>[2x]MAAQLALNSEASLWGPYREIWQTVLSALIKRQPEAVHSLDIVLKKYKPDFISLFKNPPKSAQQHERVQKASTEGIPIKGTQRTRILEEQLIKEAFILSDLYNIGEIAAVELLLIGEQQQPTFHGLTRGLVAILLYWDGKSCMAESLLHLIQARKGKTFTLDHSPEVVSMVTRFTDDLMEQGLTNKILTLISQIDVNNEFDKLKKERGLGNKKHRKEVSDLIKECQQSLAHSLYSWSCQTPLNREDTLLLIGYLEKVTVEGDGSLDKVNLTLLMSLLYCLDVGFLEQGTDDREELMKQASMFMDRQYIAAIHNRLQNTQPWKSPGMQATVRLAWALALRGISQFSEVLEFSEADEPMAEIAIGGNVFLFLTEAVVGSESFCTDEFFIRRIHKLVTDFPTLMPMKVKQLRNRAEEDARLIQMSMQMGNEPPASLRRDLEHLLLLIGELYRKDPFHLELALEYWCPTEPLQSTSLMGSFLGVAHQRPPQRQVLLSKFVRQMSDLLPATLYLPYLKMLRGLASGPQCAHYCFSLLKANGGSSAENLQAAGGSPVSWDHFFHSLMLYHEHLRRDLPNTDNIHQRHPPLRGITQRELDGLIACLQLTCTIIDWSESARLALCEHAQWMPVVVILGLLQCSIPPLLKAELLKTLAAFGKSPEIAASLWQSLEYTQILQTVRATGLRQGVGIEVELNEIESRCEEYPLTRAFCQLISTLVESSFPTNLGAGLRAPGFEPYLQFLRDTVFLRYRTRAYRRAAEKWEVAEAVLDVFYKLLKDYEPQPEDFVDQYVELQGEERVAFKPPGFSLMHHLLNESPMLELCLSLMEEGVTQLDTYAPFPGKKHLEKAVAYCFMLLNLTLQKENRFMDLLRESHLSMIVTPLEQLLQGINPRSKKADNVVNIARYLCHGNSNAELAFESAKILCSISCNSKIQEKIVGDFTQDQNVSQKLMVGFVSCLDSEEAEELLDSEKEAEDQVKQTNIRYMTKIHILNLLITSLEMKAPNLAMFLLGYELKKPVSTTNLQDSGVLGCPRTCLHSILDILRKGTDVRAGPVAVWDTPHLAELCYQVIYQLCACADTSGPTMRYLRTSQDFLFSQLQHLPFSVEESEISAMNQMSWLMKTATIELRITSLNRQRSHTQRLLHLLLDDMPTRPYSADGEGGMEDESRSLSGFLHFDTTSKVRRKILRILDSIQFSNEIPEPLQLDFFDRSQIEQVIANCEHKNRRGQTVCNVKLLHRVLVAEVNALQGMAAIGQRPLLMEEINTILQYVVERNKLLQCLHAKRHALESWRQLVEIILTACPQDLIPTEHRQLIIRDLLQDLHVKILDDDAAQELMPIVAGAVFTLTAHLSQSVRTELKQPMTASGLGQSQYVQMLDGSFAAPPGTENISAGFASIGDSSLHMILRNLLEFILKTGGGFQRVRAHLYGSLLYYLQIAQRPDEPDTLESAHKSMWERLTAPEDVFSKLQRDNLSIFESYGTALMEVVCRDACDGHDIGRMLALALLDRIVSVDRQQQWLLYLSNSGYLKVLVDSLAEDDVVLRNLLTPQPPLLKALYIYESKMAFLTRVAKSSQGAIELLRSGVIVRLAQCQVYDMRPETDPHGVFGMRETPVFIPAPVERYRQILLPALQICQLILTSSTAQHLQAAGQVLQFLVAHSDTIQAILRSQEGSLGSLQELALLTGIISKAALPGVLNELDIGLNDGSMMELQGHIGRFQRQCLALLNRFGGSDRLRQLSLQDDSSRLDGVSKKDDMELAMQQICSNVMEYCQALMIQNSPSFQQTVCLFTPSLKESASRDGTRQDSQVSILPSWRLPSLGVVIHLLKQSANNFFTYYDIHRQSVGKLQNVEQLPPDEIKELCQSEMPVGADKISTTQKYGLARRRLVKLINSRAKLLSLCSYIIETCLYILWRHLEYYLLHCTTSDSQDPVFSNMTFGNRRFQDTFNTDPNMDPRNLRQNKVSQQDVDTLLREGANSFGESLQKRLLDIESLYCKVRSRHSFIQALVRRIRGLLRVSRV;>[2x]MAAAGSLYWRTSRELWTILLGRSSMKDGYQIKAELDRYGDRLLQGLAYYKPPSTRSADKVKANKNLSPALQELGLRLSKFLALDEEQSVELLQTYLQYDYRGTQESVKVLPQDERQSQALMLKMADYYYEERISLLRCVLYILNYFQDDKHPYSAEFSKCVELMEQKELFGKYLKQFESLCREEAPTWETHGNFMTERQVSRWFVQRLREQAMLLEIIFLYFACFAASPSDLLALTKLFKEQGFGCRLQNHHLVEPSMDPLVERIGYFSILIFLEALDMDTLMTCSLSDKIEQHPFSSEEQVCKEMDSILVTLGDVPHHGPVLLAWALLRFTLNPDKVTSAVRKMGSTAIQLHLFQYLTRMLQSLRSGENNCTTSTACLCVYTFLAYVLSTLEEQVSQSQQDLVETACQVFAAPNLPDLFWNMEPTAGLGILLDSVVGMFPFRISPLLKLFTALVSKSSAKKVYSFLDRMSSYTEHYRHKPHDILSHDDETLWKRQTPKLLYALGLGQTNLRIPQGALGQVMADENGFLVRWEYSYSCWTLFTCEIEMLLHVVSTADVIHQCQRVKPIIDLVHKVISTDLSIADCLLPITSRIYMLLQRLTTVMNPPMDFLSSCVDCLTALATRLPAKVWTDLRHTGFLPFAANPVSGHLISTEGMNAGGYGSLFGIEQSQGEYSVTLSFLRLITTLVKGQLGSTQSQGLVPCILFVLREMLPNYHRWRYNSHGVREQLGFQILSLIHAILNLCPEEEEGSSAPNLRSLCIFSLTNTEAGQAVINIMGIGVDTLNTVMLTQAGSSGTEGQGQMLMQTIKLAFSITNNVIRLKPPSSGVSPLEHALTQHGAHGNNLIAVLAKYIYHRYDPSLPRLAIQLLKRLAMVAPMSVYACLGSDAAAIRDAFLSRLRDNIEDMQIKIMILEFLTVAVETQPGLIELFLNLEAKDTNEGSKEYSLGEWSCLQVVLKLIDSQDPESSWGAPLLHRSAIAFLHALWQDRRDSAMTVLRTKPNFWENLTSPLFGTLACPSESSELSILETCAFIMKIICLEIYYAVRGSLGDSLKKILKKFSEEERFTYWSNYVHSLVCQVAETEGTCNSLTEYQQLLSAWRMFLIVATHNADVMHLTNPEVRQKLFKDILGGTQALLVVPRSVACMHLSSMLCTVMIILLRRWKNDLAAPEDILNSLTQILEGVLQRDQQLVEKTKAQIFSALISVLEMKPMKASEIPQYSQLLLNVCETLQEEVVSLVDHTRHEVPASDTSEDKDSMETEDTGRIRQKDQRDGVCVLGLHLAKELCEADEEGDQWQQVLRKLPVLPILFSALEVSLRIKQNLHFCEAILHFLFTLAKTHQGAAAMAGAGITQTVCLPLLSVYQLSSNGAGSVQPAVSLRKSLDAPSWPGVYRLTVSLMERLLKTLRYNFLSEALDFVGVHQERILQCLSAVRTVQSLSCLEEADHTVGFLLQLSNFTKEWHFHLPQLIKDVQVNLCYLCQACTSLLHSRKMLQHYLQIKNGESMSSTATPRGQRTPQTPSKQPTAESEALELRQLRTVQHSLLKILGKTLATLRAFTPDLCQILQVQPLDLAQYNLLFALSFTTPAFDADVTPSFGTLLATVNVTLSMLGEMDKKKDHPLSRALVESNNTGESKNNKSLLLFIMENCFYLLISQAVRYLRDPSVHPRDKQRMKQELSSELSTLLSSLSRYFRRGGPSSPAGGLMPSPQPKGASAAKVVPEAQEPLIQLVQAFVRHVQR;>[4x]MDGEGFGELLQQAEQLAAETEGVTELPHVERNLQEIQQAGERLRSKTMTRTSQESANVKASVLLGSRGLDISHISQRLESLSAATTFEPLEPVKDTDIQGFLKNEKDNALLSAIEESRKRTFVMAEEYHRESMLVEWEQVKQRVLHTLLASGEDALDFTQESETSYISESGAPGRSSLDNVEMAYARQMYMYNEKVVSGHLQPSLVDLCTEAAERLDDKNVSDLWVMVKQMTDVPLIPASDTLKSRCSGQMQMAFVRQALNYLEQSYKNYTLISVFANLQQAQLGGVPGTYNLVRSFLNIRLPTPIPGLQDGEIEGYPVWALIYYCMRCGDLMAAQQVVNRAQHQLGDFKNCFQEYIHNKDRRLSPTTENKLRLHYRRAVRASTDPYKRAVYCIIGRCDVSDNHSEVADKTEDYLWLKLSQVCFEDEANSSPQDRLTLPQFQKQLFEDYGESHFAVNQQPYLYFQVLFLTAQFEAAIAFLFRLERTRCHAVHVALALFELKLLLKSTGQSAQLLSQEPGEPQGVRRLNFIRLLMLYTRKFEPTDPREALQYFYFLRNEKDNQGESMFLRCVSELVIESREFDMLLGKLEKDGSRKPGAIDKFTRDTKTIINKVASVAENKGLFEEAAKLYDLAKNPDKVLELTNKLLSPVVSQISAPQSNRERLKNMALAIAERYKSQGVSAEKSINSTFYLLLDLITFFDEYHAGHIDLSFDVIERLKLVPLSQDSVEERVAAFRNFSDEIRHNLSEILLATMNILFTQYKRLKGSGPTTLGRPQRVQEDKDSVLRSQARALITFAGMIPYRMSGDTNARLVQMEVLMN;>MPSATPGAPAASAAMQEALEGAGRIIDRLLQEDRAYPDLSELLNVPVHTCPTISGVSEMDYPLQSPGLLTIPSLPEISAIRRVPLPPELIEQFGHMQCNCMMGVFPEISRAWLTIDSDIFMWNYEDGGDLAYYDGLSETILSVGLVKPKTGIFQPHIRFLLVLSTPVDIVILGLSFANLQPGNLNDSISGGMQLLPDPLYSLPTDNTYLLSITSTDNGRIFLSGKDGCLYEVEYQAEAGWFSQRCRKINHSKSSLSFLVPSVLQFAFSEDDPIVQIAIDNSRNILYTRSEKGVIQVYDLGVDGHGMSRVASVSQNSLVSAAGNIARTIDRNVFKPIIHISVIEMSESVNCHLLAVTHTGVRFYFSTVPFKQPTARPCMLALVHVRLPPGFSASSNVEKPSKVHKALYNNGVLLMAASENEDNDMLWCINRDSFPFQKPMMETQVTTQVDGHSWALSAVDEQKADKIVTPLNKDLIPLTDSPVIIQQHMIPPKRFVLLSAQGSHIFYKLRPVDQLRHLLVSNSGGDGEEIERFFKLHQENQACATCLILACSSAASDREVSSWAARAFFRYGGEAQLRVQSALHAPSNVGPIFGSPLPVASPIPVGSPMPNPSFLGTPTQGACPPNVSTPAYGVATPAPQPPAVPGMMGTEIVFSGKHNGICIYFCRIIGNIWDGSVAVENTFQSGNREVTAIDSSVTPQHLESVLKELKGLLEFLDRYSQFTAGSLGNPGFGTPANRQQRLVSLGRPDIGSSQQAQQELQRKYHTEAQLAEQFSLQGIHQLVRKMCQALALWKLLCEHQFSLVVSDLQKELQEQLKITTFKDLVIRDKELTGALTASLISCYIRDNASVDGISYRLQEVCPLLYSTDDAVCSKANELLQRSRHVPNKQEKERMLRESLKEYQKISQQVDLPNVCAQYRQVRFYEGVVELCLSAAEKKDPQGLGLHFHKNGEPEEDMAGLQAFQERLNSYKCITDTLQELVNQSKAAPQSPSVPKKPGPPVLSSDPNMLSNEEAGIHFEQMLKLAQRSADELFNIALFNWLIQADLTDKLLELNSPFLEPHLVRMAKLDQNKVRYMDLLWRYYEKNRNFSNAARVVAKLADMHSPEISLKQRLEYISRAILSAKSSTTMSTLAADGEFLHELEEKLEVARIQLQIQETLTRQYSHHSTVGDAVSQLDSQLMDITKMFGQYADPFRLSECKLAIIHCAGHSDPILVQTLWQDIIDKELSDSMGNSSVDRMQSLHLKITSLGKIYASTPRYFPLEFLVKYLEQQVCNFSWDAGFVTYTMQEINVPVPKLLEVYDHLFKARDPWWSRMKKPLHLLESIYILLSGYVQEPSKVPSYERRRFTTLCLDAISCYLVELQSMDPAPALLNTVSNFKSLQAKLERLS[6x];>MAFNFGATTGTPANQGTTGFSLGTFTPKTTTSGFGFGTTTTTAPTGFGGGFGGFGATTTASTGPAFSFTTPANTTSGLFGATQNKGFGFGTGFGSTTTSTGLGTGLGTGLGFTGFNTSQQQQQQSVLGAGLFNQSFQSTPQSNQLINTASALSAPTLLGDERDAILAKWNQLQAFWGTGKGFFMNNTPPVEFTQENPFCRFKAVGFSYIPNNKDEDGLISLIFNKKESDIRGQQQQLVESLHKVLGGHQTLTVNVEGVKTKADNQTEVIIYVVERSPNGTSRRVGASALFSYFEQAHIKANMQQLGVTGAMAQTELSPVQIKQLIQNPLSGVDPIIWEQAKVDNPDP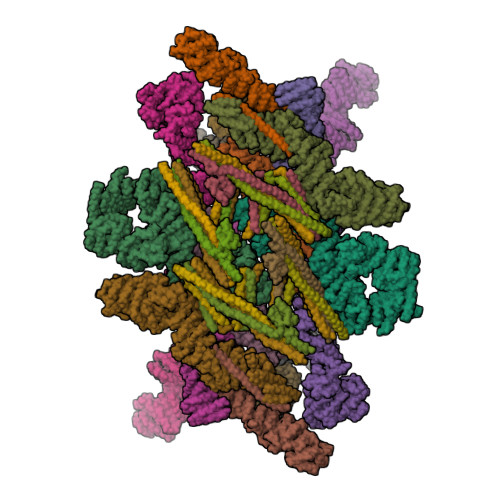ERLIPVPMIGFKELLRRLEVQDQMTKQHQSRLDIISEDIGELQKNQTTTMAKIGQYKRKLMELSHRVLQVLIKQEIQRKSGFAIQAEEEQLRVQLDTIQSELNAPTQFKGRLNELMSQIRMQNHFGAVRSEEKYYVDADLLREIKQHLKQQQEGVSHLISIIKDNHEDIKLIEQGLNDNLHMRTGFLS[4x];>[4x]MSGFNFGAASAGGFSFGNPKSTTTTAPTGFSFGAATAAPSGGFSFGTATPTPASTTGQTSGLFSFSNPAPSLAPTSGFSFGAQVTSTPAPSSGGLAFGANTSKLNSGVGNQPAGGTTQTSQPMGGFSFGAATTQTQPSATSVGGFSFAGGVGSTSTNVFAQPAASTGITLQSAVSTAAAPTATTSQPTSTFSFGTQPQAAPALNFGLLSSSSVLSTASTPAAAQPVAPTTGLSLNFGKPADTSAAVTSTGSTTTNTPSLSSLLGTSGPSLFSSVATSTVPSVVSTVASGLSLTSTATSTGFGMKTLASSAVPTGTLATSTASLGVKAPLAGTIVQANAVGSAAATGISTATAMTYAQLENLINKWSLELEDQEKHFLQQATQVNAWDRTLMQNGERITTLHREMEKVKLDQKRLDQELDFILSQQKELEDLLTPLEESVKEQSGTIYLQHADEEREKTYKLAENIDAQLKRMAQDLKEVIEHLNTSAGPGDASNPLQQICKILNAHMDSLQWIDQNSALLQRKVEQVTKECESRRKEQERGFSIAFD;>MASGFSFGTAAASTTTLNPTAAAPFSFGATPAASNTGTTGGLGFGAFNAAATPATTTATTGLGGGLFGAKPAAGFTLGGANTATATTTAASTGFSVGFNKPAGSATPFSLPVTSTSSGGLSLASALTSTPATGPSPFTLNLGSTPATTTAAATGLSLGGTLTGLGGSLFQNTNPSATGLGQSTLGQSTLGQSTLGQSLLGQSLLGQSLLGQSTLGQSTLGQSLLGQSLLGLGLNLGAVAPVSQVTTHEGLGGLDFSSSSDKKSDKAGTRPEDSKALKDENLPQLLCQDVENFQKFVKEQKQVQEEISRMSSKAMLKVQEDIKALKQLLSVASSGLQRNALAIDKLKIETAEELKNAEIALRTQKTPPGLQHENTAPADYFHTLVQQFEVQLQQYRQQIEELENHLATQSNTLHLSPQDLSMAMQKLYQTFVALAAQLQAVNENFKMLKEQYLGYRKAFLGDSTDVFEARRAEAKKWQNAPRVTTGPTPFSNIPNAAAVAMAATLTQQQQPTTGFGSSSAFGGNTSGSSSFGFGTANKPSGSLSAGFGSTSTSGFNFSNPGINASAGLTFGVSNPSSTSFGTGQLLQLKKPPAGNKRGKR[4x];>MTMLGERLVLRWRVAASFAWSVILMPVCCALFIVLSRIQILHPIQWLTDSISDLTSSYTIFCLLLICAILGLQCTFLMEYYTVVPSIPCSRLALIGNLLLPHRILHSLAHVAMGVLASWCYAVLSKGKYQLLVVSCTLQSEDEADKPSHCLNESHLFQLLCGAFFGYSYSLQYFVHNMNYLSFPSIQQYKYLQFRRFLPLIIKQSVFQSLYFIRSYAILYFCLGNIPRTWIQTALNLHMDRQQPSLDTLRGFLNLSLFYQIWLSGTFLLATWYMVWILFRIYTTEARIFPVQTSFAEEAEKCLPFILNSNTLPLVKYLAMQDLVLLSQYSPSRRQEVFSLSQPGGHPHNWTSISKECLNLMSSLTSRLIAHQEAAANNGRMRVPSSPKQIRKSSSSSGTSLIEDSAEQTQNLSTIPRIGIPSLLKTASLKSSLDIGSPFATPGVKQMSESLDPNTPCHGSVQSPQVTRRGAKLWTSDSDVQKNGSEVSPVMHRPVCNGAKQGILHTWFQHKLVQIKNVLSKRGLIMYLFSKHPEASSQDVFADAQIHIWALEALSHLVAASFSEDRMGVVQTSLSSVLAILLTLQEAVEKHFKLPHASSKPARNPGSLLDSSCKTLRFSLRAALKTAIYRITTTFGEHLHAVPVSSEHKKKLQQFLDFKE[2x];>[2x]MCSLDLFPPPLDGSQLPLYEFNNEIVAGKGFDNPPPTFQSELVNIPEPTIPVDALKAPGRMELSSKTAFIHQKESIWKRCLNAWHNVGLAGFLEEMSNSKEEVPPWLCHVTRCSLAVCRSVSSLHGSLFPHLTISPQMKSEDLTAEFSQALGWADCPLRAFAWHPHTYKFALALLDDSIRIYTAGSPTIPTLKHRLQKDVASLAWKPMCASVLAVACQSCVLVWHVDPTSLSTRPSSGCAQVLSHPGHSPVTSVCWSPKGGVLLSASPVDTAMLVWDVPTESCIPLQRVGGGGVTFLSWSPDGSKVLAATPSSVFRVWETQKWTCERWPTLQGRCQTGCWSPDGSRLLFAVKGESVIYSLCFSVSEGEAQAGVGGSQSATVVADVSEVVFTTHTGEIRVGGEIQSMCWDPSGERLAVLLKGNPEFEESQPVIAVFRTRNSPIFELLPCGFIHGRKGETPQLFQFHPGFNKGALLSQLWSSGRVNHFPFYFVNAQCPRFSPESIAVVPGNTISTANPRTLFTER> MKICLIDETGTGDGALSVLAARWGLEHDEDNLMALVLTPEHLELRKRDEPKLGGIFVDFVGGAMAHRRKFGGGRGEAVAKAVGIKGDYLPDVVDATAGLGRDAFVLASVGCRVRMLERNPVVAALLDDGLARGYADAEIGGWLQERLQLIHASSLTALTDITPRPQVVYLDPMFPHKQKSALVKKEMRVFQSLVGPDLDADGLLEPARLLATKRVVVKRPDYAPPLANVATPNAVVTKGHRFDIYAGTPV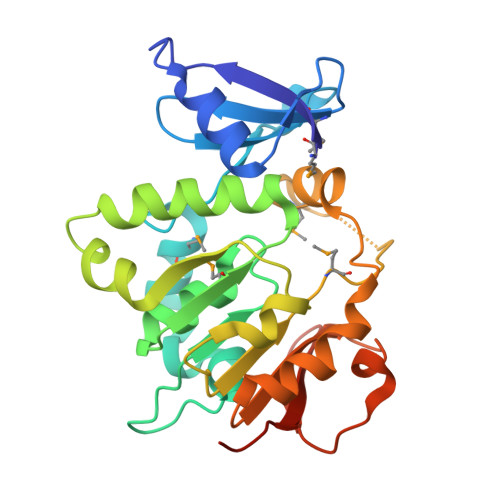LEHHHHHH> YPNASPLLGSSWGGLIHLYTATARNSYHLQIHKNGHVDGAPHQTIYSALMIRSEDAGFVVITGVMSRRYLCMDFRGNIFGSHYFDPENCRFQHQTLENGYDVYHSPQYHFLVSLGRAKRAFLPGMNPPPYSQFLSRRNEIPLIHFNTPIPR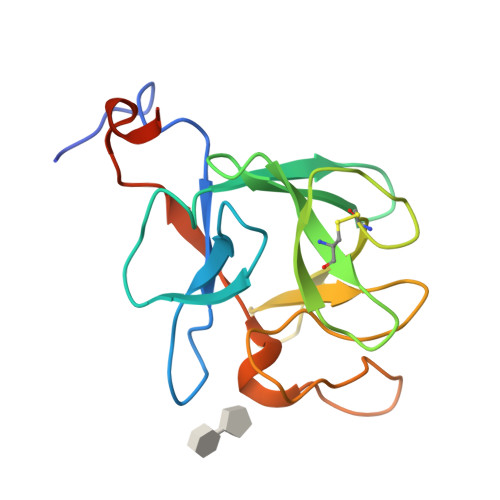RHTR> MRTSLPSPMFSRNDFSIWSILRKCIGMELSKITMPVIFNEPLSFLQRLTEYMEHTYLIHKASSLSDPVERMQCVAAFAVSAVASQWERTGKPFNPLLGETYELVRDDLGFRLISEQVSHHPPISAFHAEGLNNDFIFHGSIYPKLKFWGKSVEAEPKGTITLELLEHNEAYTWTNPTCCVHNIIVGKLWIEQYGNVEIINHKTGDKCVLNFKPCGLFGKELHKVEGYIQDKSKKKLCALYGKWTECLYSVDPATFDAYKKNDKKNTEEKKNSKQMSTSEELDEMPVPDSESVFIIPGSVLLWRIAPRPPNSAQMYNFTSFAMVLNEVDKDMESVIPKTDCRLRPDIRAMENGEIDQASEEKKRLEEKQRAARKNRSKSEEDWKTRWFHQGPNPYNGAQDWIYSGSYWDRNYFNLPDIYLEHHHHHH

Members of the OSBP/ORP family vary in length: the short ORPs contain primarily a conserved OSBP-related domain (ORD) that can bind and transfer lipids such as sterols, PIPs or phosphatidylserine (PS), whereas the long ones often possess additional functional domains for ligand binding and/or membrane targeting. The OSBPL1A gene (homo sapiens) encodes two proteins: the long isoform ORP1L (residues 1–950) containing the ANK (ankyrin repeat) domain, the PH (Pleckstrin homology) domain, the FFAT (diphenylalanine in an acidic tract) motif and the ORD, and a short isoform ORP1S (residues 514–950) containing only the ORD. Here, while we cannot rule out its cholesterol sensor function, our structural, biochemical and cell biological data suggest that ORP1L is a bona fide cholesterol transporter. Here, our results suggest that ORP1 is a unique sensor of lysosomal PI-bisphosphates, and that PI(4,5)P2/PI(3,4)P2 allosterically regulates cholesterol transport by ORP1.

To further illustrate the mechanisms underlying cholesterol transport by ORP1-ORD, we solved two crystal structures of ORP1-ORD (524–950 or 534–950) in complex with cholesterol. The most striking feature is that their N-terminal loops (residues 514–546) and lid regions (547–565) adopt different open conformations, distinct from the closed conformations observed in yeast Osh structures. To accomplish the lipid transport function, the ORP/Osh proteins were expected to adopt the open state when extracting lipids from or unloading them onto the membrane, and the closed state when transporting lipids between two membranes. Therefore, the open conformations of ORP1-ORD may represent certain important states when ORP1 exerts physiological functions (see below). The 2Fo-Fc map revealed continuous electron density for cholesterol, which binds deeply into the central tunnel in the core. In the 2.6 Å structure, the 3-hydroxyl group of cholesterol forms direct or water-mediated hydrogen bonds with Tyr583 and Gln724 at the bottom of the binding tunnel. The rigid, fused four-ring backbone and the hydrocarbon tail tightly bind to multiple hydrophobic residues at the tunnel wall. The hydrocarbon tail of cholesterol also forms hydrophobic contacts with Ile557 and Met559 in the lid region, as well as Ile549 from the lid of a symmetry-related molecule. Consistently, structural analyses of the open cholesterol-bound ORP1-ORD revealed domain swapping between symmetry-related molecules, effectively generating dimers or trimers. We thus constructed a model of ORP1-ORD monomer based on the 2.6 Å cholesterol-bound structure and performed molecular dynamics (MD) simulation. Significantly, the lid moves toward the tunnel entrance within 20 ns, and the monomeric ORP1-ORD conformations throughout the remaining simulation are similar to the crystal structures of closed Osh proteins.>MRGSHHHHHHGSMPVAGSELPRRPLPPAAQERDAEPRPPHGELQYLGQIQHILRCGVRKDDRTGTGTLSVFGMQARYSLRDEFPLLTTKRVFWKGVLEELLWFIKGSTNAKELSSKGVKIWDANGSRDFLDSLGFSTREEGDLGPVYGFQWRHFGAEYRDMESDYSGQGVDQLQRVIDTIKTNPDDRRIIMCAWNPRDLPLMALPPSHALCQFCVVNSELSCQLYQRSGDMGLGVPFNIASYALLTY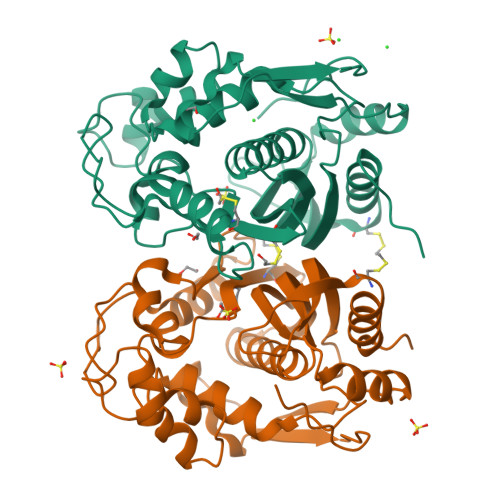MIAHITGLKPGDFIHTLGDAHIYLNHIEPLKIQLQREPRPFPKLRILRKVEKIDDFKAEDFQIEGYNPHPTIKMEMAV[4x]(8S,11S,14S)-14-{[(2S)-4-amino-2-{[2-(4-tert-butylphenyl)-4-methylpyrimidine-5-carbonyl]amino}butanoyl](methyl)amino}-3,18-bis(2-aminoethoxy)-N-[(2Z)-2-iminoethyl]-11-methyl-10,13-dioxo-9,12-diazatricyclo[13.3.1.1~2,6~]icosa-1(19),2(20),3,5,15,17-hexaene-8-carboxamide 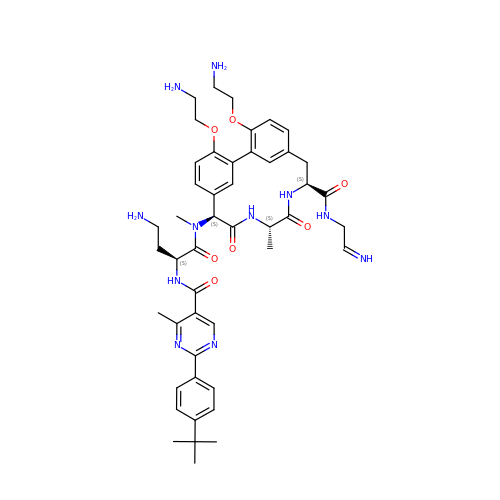| C47 H61 N11 O7 | SJYWASAPFZIDQL-UAKBWTGGSA-N>MKIEDYRLLITLDETKTLRKAAEILYISQPAVTQRLKAIENAFGVDIFIRTKKQLITTTEGTMIIEHARDMLKRERLFFDKMQAHIGEVNGTISIGCSSLIGQTLLPEVLSLYNAQFPNVEIQVQVGSTEQIKANHRDYHVMITRGNKVMNLANTHLFNDDHYFIFPKNRRDDVTKLPFIEFQADPIYINQIKQWYNDNLEQD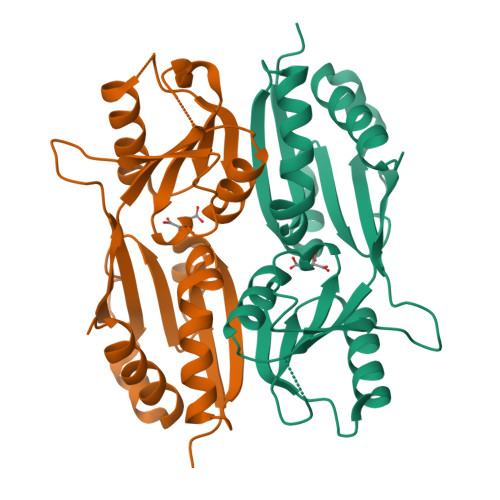YHATITVDQVATCKEMLISGVGVTILPEIMMKNISKEQFEFEKVEIDNEPLIRSTFMSYDPSMLQLPQVDSFVNLMASFVEQPKA[6x]>MRPESKKTVSAPKETTPTSTSVQTYVKENYTAKNGLIVDYKNAQEPHYLAESIGLYMEYLVEVNDSKTFQEQVSHLEKNFITEDNFIKWEATDATTTNAIVDDFRITEALYQASEKFSFPSYKKMADKILANTKKYSAEQGVPVDFYDFVHKKKADTLHLSYLNIQA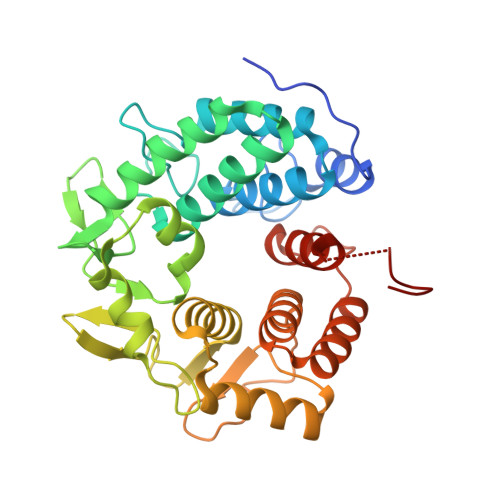MQQINYRDKAYLPIQTVNADPFFTEVFQNEQFQYADPSEVNMIDQMLIAMAYFDENGDVEPNFDNFLQTELASKGKVYARYQRETKKPSSENESTAVYAFLTQYFNKTNQAKNGKITKELLEKMDTSNPETTHFFDYINKEITLKKKLAAALEHHHHHH[2x]>MSEQKQDVAATEEQQPVLQIQRIYVKDVSFEAPNLPHIFQQEWKPKLGFDLSTETTQVGDDLYEVVLNISVETTLEDSGDVAFICEVKQAGVFTISGLEDVQMAHCLTSQCPNMLFPYARELVSNLVNRGTFPA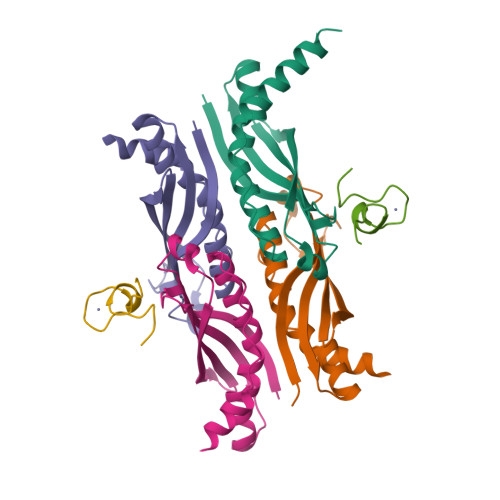LNLSPVNFDALFVEYMNRQQAENAEEKSEEEQTKH[8x];>RIGRNEPCPCGSGKKYKHCHGSRVARQ[2x]>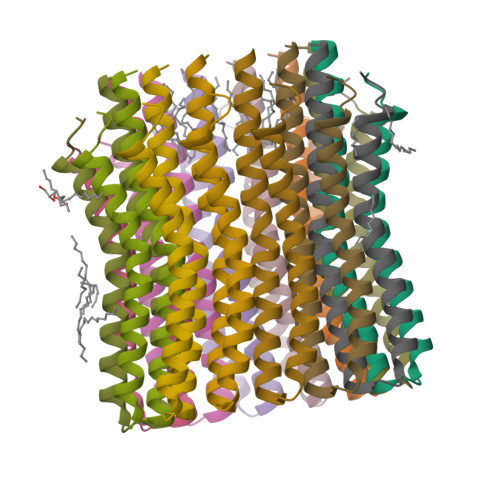MNPLIAAASVIAAGLAVGLASIGPGVGQGTAAGQAVEGIARQPEAEGKIRGTLLLSLAFMEALTIYGLVVALALLFANPFV[14x]1-(6-bromo-5-ethoxypyridin-3-yl)-1,4-diazepane 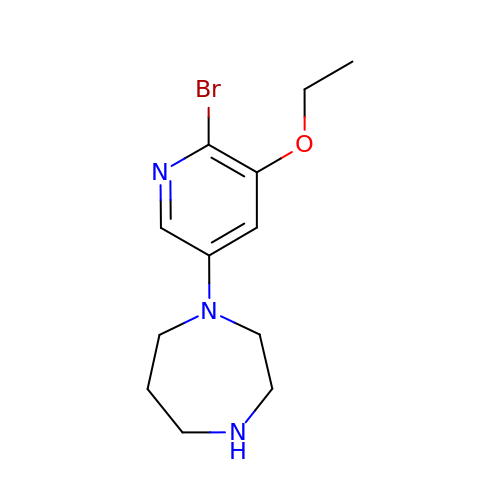| C12 H18 Br N3 O | UGNNTIXQGYYUAP-UHFFFAOYSA-N> ILGGREAEAHARPYMASVQLNGAHLCGGVLVAEQWVLSAAHCLEDAADGKVQVLLGAHSLSQPEPSKRLYDVLRAVPHPDSQPDTIDHDLLLLQLSEKATLGPAVRPLPWQRVDRDVAPGTLCDVAGWGIVNHAGRRPDSLQHVLLPVLDRATCNRRTHHDGAITERLMCAESNRRDSCKGDSGGPLVCGGVLEGVVTSGSRVCGNR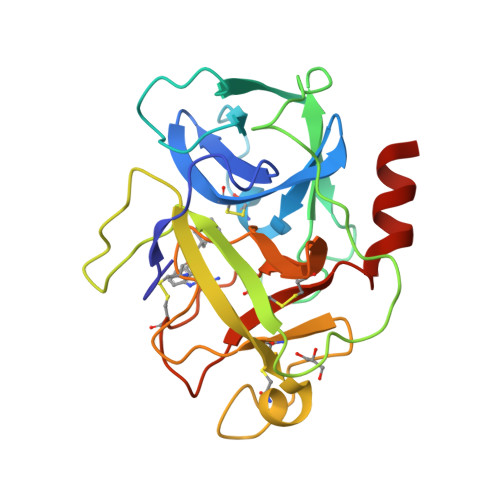KKPGIYTRVASYAAWIDSVLASAAA>MIICSVDIGIKNPAYAIFNYDNTSNTIKLIAIEKSDWTKNWERSVARDLTRYNPDVVILEKQGFKSPNSKIIYFIKGFFYNSNTKVIVRNPTFKGGSYRNRKKQSIDVFIQKISEYTDYKNDILNKYTKLDD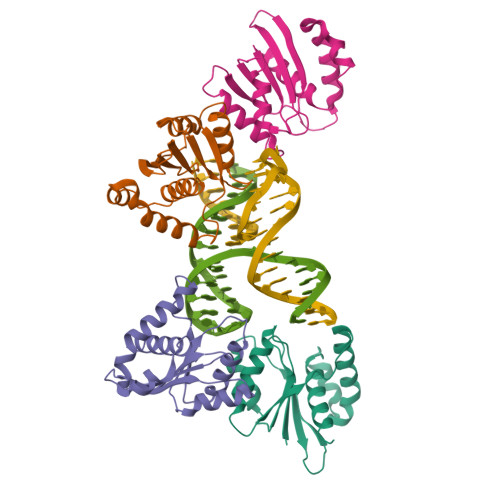IANSFNLGLSYMESLLK[4x]>[6x]GSMAKGNGLLYGKRGLILGLANNRSIAWGIAKTASSAGAELAFTYQGEAMKKRVEPLAEEVKGFVCGHCDVSDSASIDAVFNTIEKKWGKLDFLVHAIGFSDKEELSGRYVDISESNFMMTMNISVYSLTALTKRAEKLMSD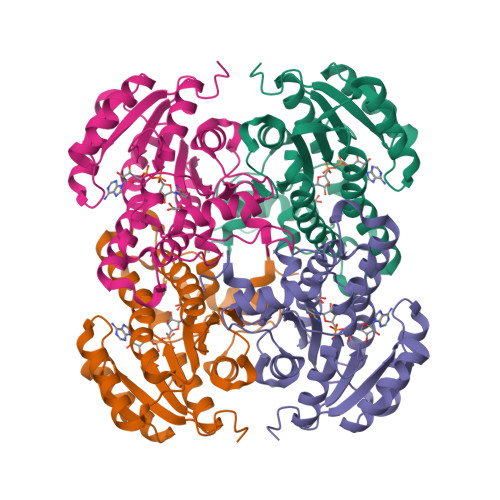GGSILTLTYYGAEKVVPNYNVMGVAKAALEASVKYLAVDLGPKHIRVNAISAGPIKTLAASGIGDFRYILKWNEYNAPLRRTVTIEEVGDSALYLLSDLSRSVTGEVHHVDSGYNIIGMKAVDAPDISVVKE> GPGSEDLPLPPGWSVDWTMRGRKYYIDHNTNTTHWS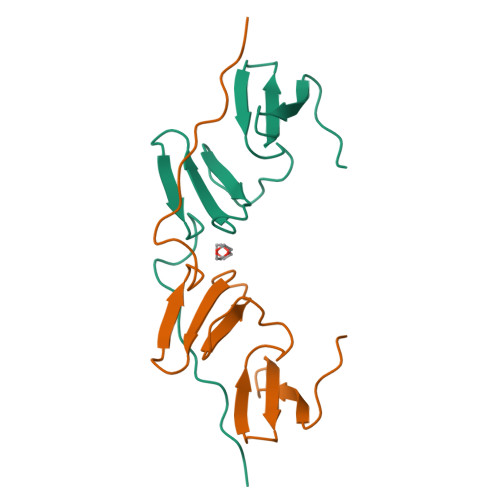HPLEREGLPPGWERVESSEFGTYYVDHTNKRAQYRHPCAPSVPRYDQPPPITYQPQ>CCAGGCCTGG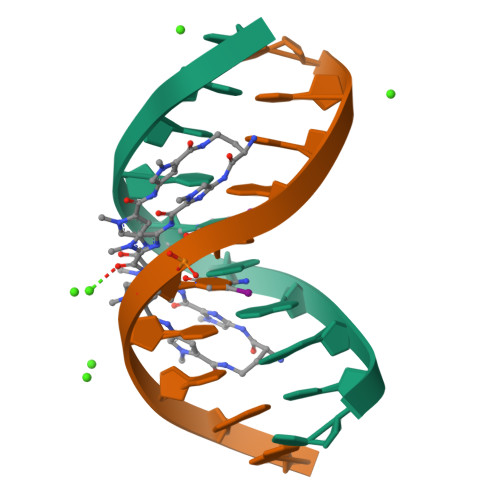[2x]>[2x]MHHHHHHLPNITILATGGTIAGGGDSATKSNYTVGKVGVENLVNAVPQLKDIANVKGEQVVNIGSQDMNDNVWLTLAKKINTDCDKTDGFVITHGTTTMEETAYFLDLTVKCDKPVVMVGAMRPSTSMSADGPFNLYNAVVTAADKASANRGVLVVMNDTVLDGRDVTTTNTTDVATFKSVNYGPLGYIHNGKIDYQRTPARKHTSDTPFDVSKLNELPKVGIVYNYANASDLPAKALVDAGYDGIVSAGVGNGNLYKSVFDTLATAAKTGTAVVRSSRVPTGATTQDAEVDDAKYGFVASGTLNPQKARVLLQLALTQTKDPQQIQQIFNQY

L-asparaginases catalyze the hydrolysis of L-Asn to L-Asp. The genome of E. coli encodes three L-asparaginases, called type I, II, and isoaspartyl aminopeptidase/L-asparaginase, respectively. The active site pockets of these enzymes are shaped by two protomers, one of which forms most of the active site scaffold, including all catalytic residues; it will be referred to as a “major” protomer, with the second protomer called “minor”. Yet, as we demonstrated here based on the reinterpreted structures of EcAI and the new structures of EcAII, under some conditions a citrate ion can be accommodated into the active site cavity and even displace the canonical substrate or product.

Three structures included in this report, referred to as EcAIID90T/K162T-L-Asn50, EcAIID90T/K162T-L-Asn56, and EcAIID90T/K162T-L-Asn62, were determined for crystals of the EcAIID90T,K162T variant grown in the presence of 10 mM L-Asn at pH 5, 5.6 and 6.2, respectively. All three structures, refined at the resolution of 2.15 Å or higher, are isomorphous and belong to the space group P3121 with two protomers, representing half of the biological assembly, present in the asymmetric unit. We found that the structures are practically invariant within the pH range explored in this study, both in terms of the overall fold as well as details within the active site region. Therefore, we will describe only the structure of EcAIID90T/K162T-L-Asn50. Somewhat unexpectedly, we found that in all three structures one of two independent active sites (in protomer B) was occupied by a citrate anion, despite the fact that L-Asn was present in the crystallization buffer, which is illustrated in Fig. S2c. The position of the citrate in these structures differs significantly from those observed for EcAIIwt-apo7 or for complexes of EcAI. In this case the ligand is stabilized by interactions with the affinity His6-tag, contributed by a symmetry-related protomer, therefore the observed binding mode is an experimental artifact. Under these conditions, a citrate anion is partly (pH 5.6 and 6.2) to predominantly (pH 5.0) mono-protonated on β-carboxylate, with a significant contribution of the doubly-(β1/β2)-protonated form at pH 5.0. Although three conserved interactions described earlier for the α-carboxylate group of citrate are not preserved, this moiety still forms two H-bonds with Ser58, indicating importance of this residue for ligand binding.>MKFAEHLSAHITPEWRKQYIQYEAFKDMLYSAQDQAPSVEVTDEDTVKRYFAKFEEKFFQTCEKELAKINTFYSEKLAEAQRRFATLQNELQSSLDAQKESTGVTTLRQRRKPVFHLSHEERVQHRNIKDLKLAFSEFYLSLILLQNYQNLNFTGFRKILKKHDKILETSRGADWRVAHVEVAPFYTCKKINQ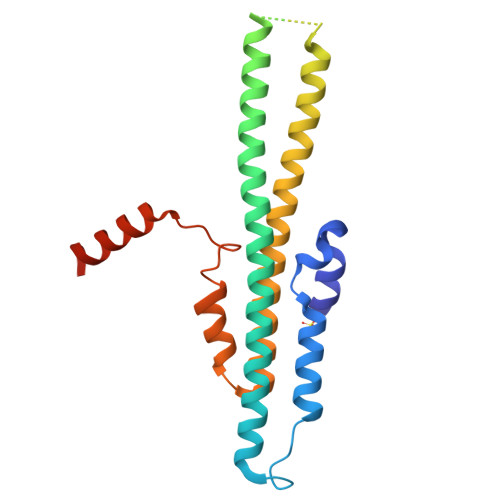LISETEAVVTNELEHHHHHH[2x]The cytochrome bc 1 complex, also known as respiratory complex III (CIII), in the electron-transfer chain of the inner mitochondrial membrane is a homodimer (CIII2) of two biochemically identical protomers. CIII2 catalyses the transfer of electrons from the lipophilic two-electron donor ubiquinol (QH2) to the water-soluble, one-electron acceptor protein cytochrome c, contributing to an electrochemical proton gradient across the membrane. Electron transfer within the complex occurs through the prosthetic groups of the three catalytic core subunits: heme b L and heme b H of cytochrome b (cyt b), heme c 1 of cytochrome c 1 (cyt c 1) and the [2Fe–2S] cluster of the iron–sulfur protein (ISP), often called the Rieske protein after its discoverer. The Rieske domain is tethered to the complex by one transmembrane helix and a connecting flexible linker that acts as a hinge.

The [2Fe–2S] cluster can thus be positioned close to the Qo site (referred to here as the b or proximal position), which is formed by cyt b. The Rieske domain approached the Pf-type inhibitor-induced structure most closely when the high-potential chain was reduced by sodium ascorbate, with a similar hydrogen-bonding distance between the Rieske domain and cyt b. Density inside the Qo site was weak, suggesting that no substrate had remained bound during sample preparation. The Fe–S cluster-bearing tip of the Rieske domain was well-resolved in the two ascorbate-reduced samples. Density at the hinge, where the transition from helix to random coil occurs with Pf-type inhibitors bound, and density distal to the tip was weak, indicating heterogeneity in these regions. A shift towards the b position in the equilibrium of positions was not observed. Consistent with previous EPR experiments, the Rieske domain was found in a position closer to cyt b when the high-potential chain was reduced by sodium ascorbate compared with when it was fully or partially oxidized. Despite the closer interaction of the Rieske domain with cyt b, no shift in the equilibrium of positions in ascorbate-reduced samples was observed. Together with the weak density in the hinge region between the Rieske and transmembrane domains in these samples, this may indicate that the close interaction of the cluster-bearing tip with cyt b loosens the helical secondary structure of the hinge only transiently.

>[2x]MNSLLRLPALKRGVFTMSKRGLATTVSPKTRTSNLKNGLTIASESNPLVQTATVGVWIDAGSRNENAYNNGTAHFFEHLAFKGTDKRSQHQLELDIENMGGHLNAYTSRESTVYYAKSFKDDVPKSVEILADILQHSKLAESAIDREREVITRELEEVNKQYEEVVFDHLHATAFMNQPLGRTILGPRENIQTITNTELRKFITENYTADRMVLVGAGAVDHDALVELAEKYFSHLPSSQSPVPLGTPRSSGEDANQNPIPNFVGSEVRLRDDTMPVAHIAIAVEGVSWTSEDYYTALVAQAIIGNYDRAVGTSRHQGSRLSNIVSENNLANSFQSFSTSYSDTGLWGIYLTSENTTQIDDLVHFTLKEWNRLSTSVSNLQVERAKSQLKAGLLLSLDGTTYVAEDIGRQLTTLGRRVTPAEVEAKLEAVTEHDVRAWAQKTLYDKDIALVGLGPIEGLYDYNRIRNDMSMMRW;>MTRGVPRLAVAARHFSTAEAAGVKVAAQDGQSPISDLSVVLRGGSRYATVPGVSHILEKFAFQNTVPKSALRFVRELELFGGKLYTHTTREHIVLRTQFLKQDLPYFVDAFANVLKETKFQQFELTERVAPVAELDLLKRESDPAFTALEAAHEVAFRTGLGNSVYAQGYSPVTLEDVKEFARQVYAKQNVAVVGNNVVPADLQQLVGTAFADLQEGSKVTQAGTTTLHGGEARVRTSTGNALTIALPIAEPKPVYHALASFLGGPASMPWSVGASPLAQATVGTHTSVKATYHNYGDAGLFAITIKGDSPAEISQVAHKAVQALKDTGAEVTEEQAARAYAKSKFAAAEAFENPDSSASVIGMELLSGVSRIAPENVQKFTPAELSEAAAQLSASAKPVVAAVGQVHALPFADELF[2x];>MALRKKNSLLNMANSYVLDSPQPSNLNYFWNFGSLLALCLVIQLATGITLAMHYTSHASLAFDSVEHIMRDVNFGWFIRYAHANTASFFFICIYAHMGRNIYYGSYKTPRVLPWSIGVIIFLLLIITAFMGYVLVFGQMSLWGATVICNLVSAIPWLGEDIVHFLWGGFSVGNPTLQRFFALHYLMPFVLAVFALLHLIALHTAGSSNPLGITSNVDKLSMHPYYSFKDLITVFAFLLMFTLFVFFSPDKLGHPDNYIPANPMVTPASIVPEWYLLPFYAILRAIPDKLGGVIAMVAAILILLILPIVDRSIIRGNAFKPISKLLFGFFICNFLLLGVLGQVHIEPPFIVLGQICTIFYFSYFLILLPMVSTIENIFFYIGSLRK[2x];>MRRRRIGVWPENRRVSRLWVSLSPRSCVTCPVPTNQNPPINNHHTPILTQMFKAIPLRQALLGISSAVCAGATTTYYYTTKAEAMTAAEHGLHPAEYPWPQNGMLSTFDHASLRRGYQVYKEVCAACHSLDRIAWRNLVGVTHTTDEAKAFAEELEYDDEPDDEGNPRKRPGKLADYIPGPYPNEQAARAANQGALPPDLSLIAKARHGGADYIFALLTGYPDEPPAGVVLAPGMNYNPYFPGGGIGMARTLFDGVVEYEDGTPATTSQMAKDVAAFLTWAAEPEHDERKKLGLKAIIVISAMLGLSVYIKKFKWSPIKNRKFIYNPPKN[2x];>[2x]MSLLRTAAQAVKAPKAYTPLVAAKAFAQTRSVSSQPIGGKSTYKIPDFTPYLKKDRNTDANRLFSYFMIGSFGMLSAAGAKATVQDFLSNMSASADVLAMAKVEVKLGAIPLGKNVIIKWRGKPIFIRHRTSEEIEEANEVNVATLRDPQTDDERVQKPEWLVMIGVCTHLGCVPIGEAGDFGGWFCPCHGSHYDISGRIRRGPAPLNLEIPEYDFADAETLVIG;>[2x]MSYFLTLASEVAESLLPTVAFASEEEKEQDEPVEVESDDDESEEKEDDDEEEDEDDDDDDDDDEVPDPAIALHEAAAEGPCHDFKHHFDECVERVTKAQEAEDYDHAEYKEDCVEEFFHLQHCINDNTADKLFRVLK;>[2x]MASITSVVKTSELILKSPLLSKIVVPLAKTYVKFSGYRQLGFKMNDLIIEETPNMQLALRRLPPTESYDRVYRLIRATQFSLSHKLATGNDITKPEEDDHYLIPYILDVEAEAFEKDALDNLEVVKRK;>MGGNGHYMGWWGHMGSPPQKGIAGYTISPFAARPFAGVVHAAIFNTFRRTKNQALFVILPVSFFYYVWTQASEKNEWLYTKAGRHELAKALAE[2x];>MAWATTFYNVFVKRNSAFVATILASAFVFDMTFETAIDNFWDRINAGKQWKDIRHKYIEAAGDDDEDDE[2x];>[2x]MICGEGDYVKKPSYKIVPHFLGFNIPTVSKWIPIFGIWGAAAGIGALFLIEGVPRTRQDILSKIPIIGEHWIREIPASDNPF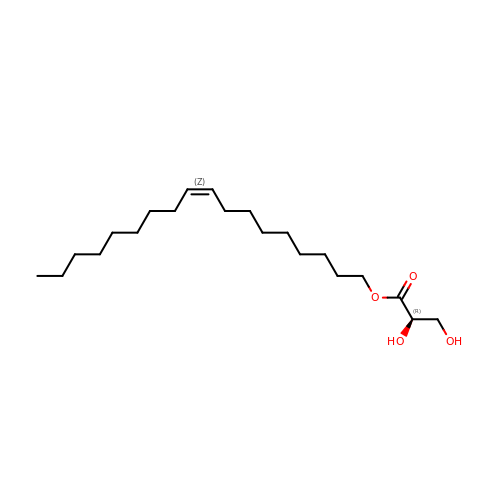[(Z)-octadec-9-enyl] (2R)-2,3-bis(oxidanyl)propanoate | C21 H40 O4 | JPJYKWFFJCWMPK-GDCKJWNLSA-N RJ contains 12–15% protein, of which 82–90% are members of the major royal jelly protein family (MRJPs) that share high homology, and are designated MRJP1−95–7. Besides their nutritional role, MRJP1 is a key factor responsible for honeybee development. Interestingly, the MRJP1 oligomer reportedly comprises both MRJP1 and apisimin. Apisimin is a serine-valine-rich peptide exclusively found in honeybee and has the tendency to form oligomers.

Because, the sequence homology between MRJP1 and any other protein of known three-dimensional structure was <17%, the structure were determined by combining multiple isomorphous replacement and molecular replacement methods, and refined to a resolution of 2.65 Å in space group of H32, with an Rwork of 23.9% and an Rfree of 27.5%. The asymmetric unit contains two MRJP1, two apisimin, four unexpected 24-methylenecholesterol (ostreasterol, Osl), and 144 water molecules. The overall complex adopts an H-shaped structure with approximate height, width, and length of 100 × 50 × 115 Å, respectively. It has an apisimin-dependent dimerisation of MRJP1 dimers quaternary structure, comprising 16 molecules, including four MRJP1, four apisimin, and eight 24-methylenecholesterol molecules. MRJP1 is folded into a unique six-bladed β-propeller shape containing 31 β-strands and 11 α-helices with a central channel. Three disulfide bonds (Cys132–Cys195, Cys118–Cys150, and Cys329–Cys416) were observed in MRJP1, with the last one stabilising the C-terminal portion. Each apisimin molecule in the asymmetric unit contains two α-helices connected by a loop, with two hydrogen bonds and a large hydrophobic zone between the two α-helices, giving apisimin a relatively stable 47° oblique structure. For the inner two Osl molecules, each is totally enveloped by two MRJP1 molecules, one apisimin, and the other three Osl molecules. Apisimin functions as a dimer joining the protein complex, stabilising the complete MRJP14-apisimin4-Osl8 tetramer. Interestingly, electron density for N-acetylglucosamine (NAG) was observed at glycosylation site Asn144 in the crystal structure.

>[2x]MTRLFMLVCLGIVCQGTTGNILRGESLNKSLPILHEWKFFDYDFGSDERRQDAILSGEYDYKNNYPSDIDQWHDKIFVTMLRYNGVPSSLNVISKKVGDGGPLLQPYPDWSFAKYDDCSGIVSASKLAIDKCDRLWVLDSGLVNNTQPMCSPKLLTFDLTTSQLLKQVEIPHDVAVNATTGKGRLSSLAVQSLDCNTNSDTMVYIADEKGEGLIVYHNSDDSFHRLTSNTFDYDPKFTKMTIDGESYTAQDGISGMALSPMTNNLYYSPVASTSLYYVNTEQFRTSDYQQNDIHYEGVQNILDTQSSAKVVSKSGVLFFGLVGDSALGCWNEHRTLERHNIRTVAQSDETLQMIASMKIKEALPHVPIFDRYINREYILVLSNKMQKMVNNDFNFDDVNFRIMNANVNELILNTRCENPDNDRTPFKISIHL;>MSKIVAVVVLAAFCVAMLVSDVSAKTSISVKGESNVDVVSQINSLVSSIVSGANVSAVLLAQTLVNILQILIDANVFA[2x]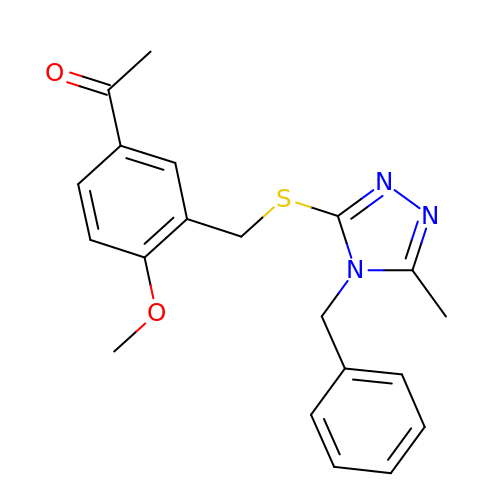1-[4-methoxy-3-[[5-methyl-4-(phenylmethyl)-1,2,4-triazol-3-yl]sulfanylmethyl]phenyl]ethanone | C20 H21 N3 O2 S | GBQPKTFARABQAW-UHFFFAOYSA-N> TAWYANXE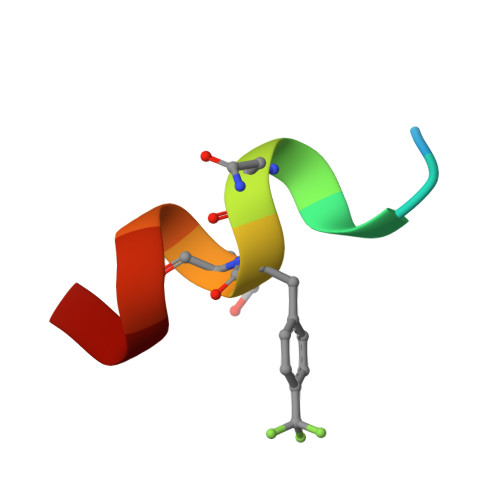KLLR>MRGSHHHHHHTDPIMKPENKLPVLDLISAEMKTVVNTLQPDLPPWPATGTIAEQRQYYTLERRFWNAGAPEMATRAYMVPTKYGQVETRLFCPQPDSPATLFYLHGGGFILGNLDTHDRIMRLLASYSQCTVIGIDYTLSPEARFPQAIEEIVAACCYFHQQAEDYQINMSRIGFAGDSAGAMLALASALWLRDKQIDCGKVAGVLLWYGLYGLRDSVTRRLLGGVWDGLTQQDLQMYEEAYLSNDADRESPYYCLFNND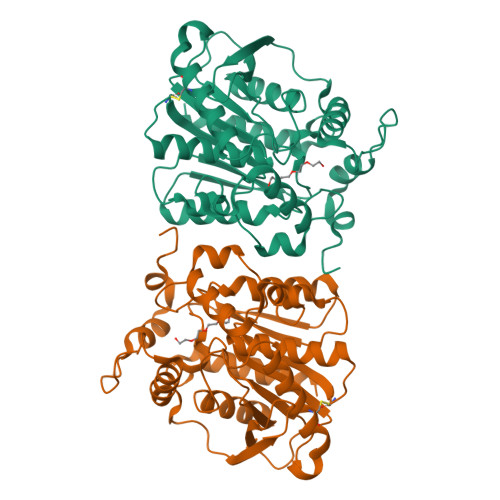LTREVPPCFIAGAEFDPLLDDSRLLYQTLAAHQQPCEFKLYPGTLHAFLHYSRMMKTADEALRDGAQFFTAQL[3x]> GDPVEDIIHDALGSTARRAISSVTNAESAANTTPSSHRLETGRVPALQAAETGATSNATDENMIETRCVVNRNGVLETTINHFFSRSGLVGVVNLTDGGTDTTGYATWDIDIMGFVQLRRKCEMFTYMRFNAEFTFVTTTKNGEARPYMLQYMYVPPGAPKPTGRDAFQWQTATNPSVFVKLTDPPAQVSVPFMSPASAYQWFYDGYPTFGQHPETSNTTYGLCPNNMMGTFAVRVVSREASQLKLQTRVYMKLKHVRAWVPRPIRSQPYLLKNFPNYDSSKITNSARDRSSIKQANM;> SPSVEACGYSDRVAQLTVGNSSITTQEAANIVLAYGEWPEYCPD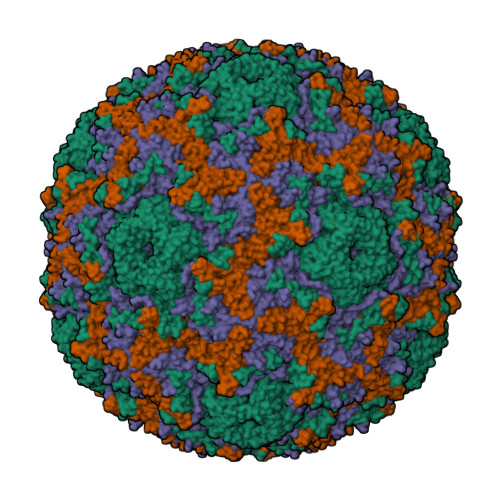TDATAVDKPTRPDVSVNRFYTLDSKMWQENSTGWYWKFPDVLNKTGVFGQNAQFHYLYRSGFCLHVQCNASKFHQGALLVAVIPEFVIAGRGSNTKPNEAPHPGFTTTFPGTTGATFHDPYVLDSGVPLSQALIYPHQWINLRTNNCATVIVPYINAVPFDSAINHSNFGLIVIPVSPLKYSSGATTAIPITITIAPLNSEFGGLRQAVSQ;> GIPAELRPGTNQFLTTDDDTAAPILPGFTPTPTIHIPGEVHSLLELCRVETILEVNNTTEATGLTRLLIPVSSQNKADELCAAFMVDPGRIGPWQSTLVGQICRYYTQWSGSLKVTFMFTGSFMATGKMLVAYSPPGSAQPANRETAMLGTHVIWDFGLQSSVSLVIPWISNTHFRTAKTGGNYDYYTAGVVTLWYQTNYVVPPETPGEAYIIAMGAAQDNFTLKICKDTDEVTQQAVLQ;> MGAQVSTQKSGSHETGNVATGGSTINFTNINYYKDSYAASATRQDFTQDPKKFTQPVLDSIRELSAPLN> MSIATIVPENA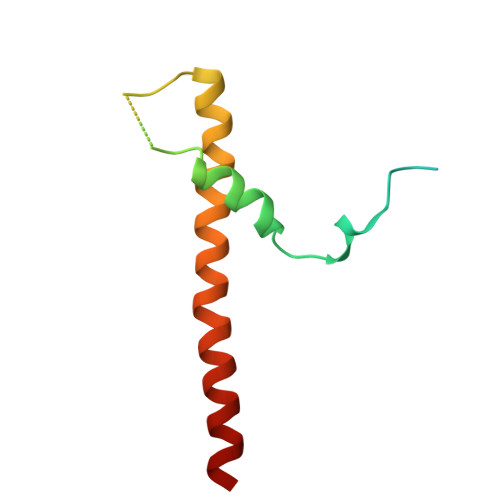VIGQAVNIRSMETDIVSLDDRLLQAFSGSAIATAVDKQTITNRIEDPNLVTDPKELAISQEMISDYNLYVSMVSTLTRKGVGAVETLLRS> MIHNYAILIVTAAVVVWYYYKLYVVDKNGKKSLVRTRKHRNLESAARR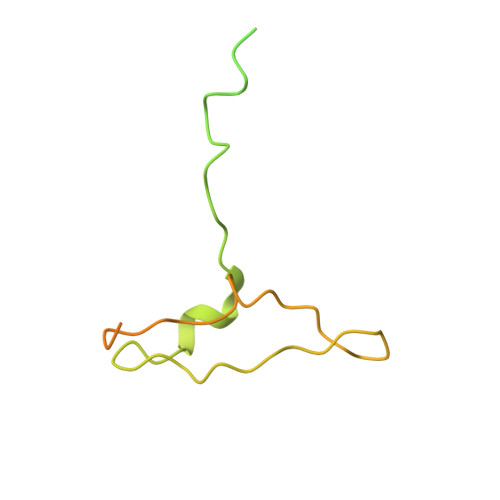DPILKTYSKQDGTRSRKPKSTKKEPHWMDPQLMGSQTTQYSRNRGYGDPIRGDLPIVPDDGGWFATRANPAHHLHTGALSMIGGDASDCGSTAVQQLIKKYEDKGCNNNGLNVMSSHYGGVM> GPGTMASVPASRYLTDMTLEEMSREWSMLIPKQKVAGPLCIRMDQAIMDKN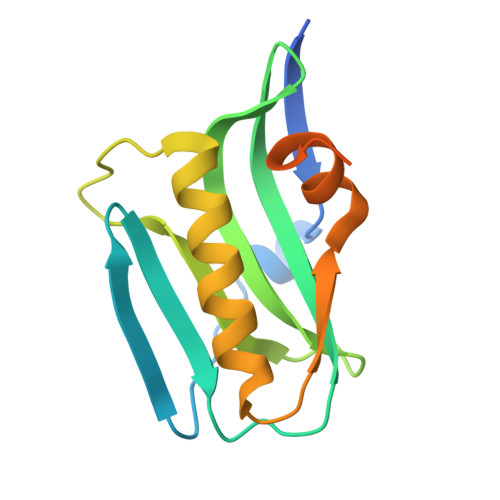IILKANFSVIFDRLETLILLRAFTEEGAIVGEISPLPSLPGHTAEDVKNAVGVLIGGLEWNDNTVRVSETLQRFAWRSSNENGRPPLTPKQKREMAGTIRSEV>ASMKIVVITEKPFAENAVKGIREILEKAGHEVVMIEKYKKKEDVIERIKDADGVIVRSDKIDEEIIKAGEKVKIIVRAGAGYDNIDIEACNQGKIVVMNTPGQNRNGVAELCIGMMIFGFRKGFKEGKGRELKDKTLGICGCGYVGKRVKEIAEGIGMKIKVYDPFITTENQVKKIEELFEECQVISLHLPLTKETKGKIGYELIKKLPYGGMICNTARKEIIDEEGLIRIMREREDLIYITDVAPTSKVFNNEFK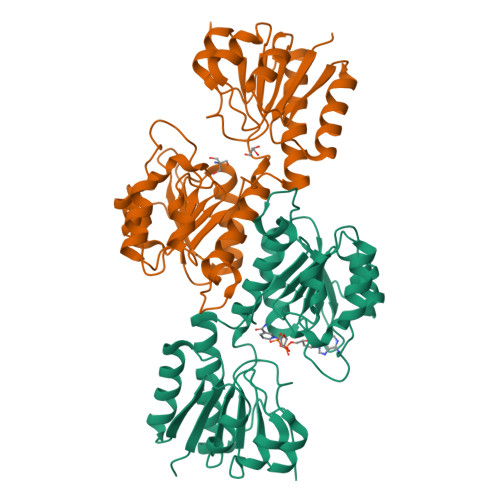GRFFATPIKIGAETEESNINAGMAAASQICDFFTNGTVKFQVNKFLEHHHHHH[2x]> MSSNRVLDLFKPFESFLPEVIAPERKVPYNQKLIWTGVSLLIFLILGQIPLYGIVSSETSDPLYWLRAMLASNRGTLLELGVSPIITSSLIFQFLQGTQLLQIRPESKQDRELFQIAQKVCAIILILGQALVVVMTGNYGAPSDLGLPICLLLIFQLMFASLIVMLLDELLSKGYGLGSGISLFIATNIAEQIFWRAFAPTTVNSGRGKEFEGAVIAFFHLLAVRKDKKRALVEAFYRTNLPNMFQVLMTVAIFLFVLYLQGFRYELPIRSTKVRGQIGIYPIKLFYTSNTPIILQSALTSNIFLISQILFQKYPTNPLIRLIGVWGIRPGTQGPQMALSGLAYYIQPLMSLSEALLDPIKTIVYITFVLGSCAVFSKTWIEISGTSPRDIAKQFKDQGMVINGKRETSIYRELKKIIPTAAAFGGATIGALSVGSDLLGTLGSGASILLATTTIYGYYEAAAKEGGFTKNLVPGFSDLM;> MSSPTPPGGQRTLQKRKQGSSQKVAASAPKKNTNSNNSILKIYSDEATGLRVDPLVVLFLAVGFIFSVVALHVISKVAGKLF;> MARASEKGEEKKQSNNQVEKLVEAPVEFVREGTQFLAKCKKPDLKEYTKIVKAVGIGFIAVGIIGYAIKLIHIPIRYVIV;> GGSGGSGGSGGSGGSPTNYEYDEASETWPSFILTGLLMVVGPMTLLQIYQIFFGANAEDGNSGKSKEFNEEVFKNLNEEYTSDEIKQFRRKFDKNSNKKSKIWSRRNIIIIVGWILVAILLQRINSNDAIKDAATKLFDPYEILGISTSASDRDIKSAYRKLSVKFHPDKLAKGLTPDEKSVMEETYVQITKAYESLTDELVRQNYLKYGHPDGPQSTSHGIALPRFLVDGSASPLLVVCYVALLGLILPYFVSRWWARTQSYTKKGIHNVTASNFVSNLVNYKPSEIVTTDLILHWLSFAHEFKQFFPDLQPTDFEKLLQDHINRRDSGKLNNAKFRIVAKCHSLLHGLLDIACGFRNLDIALGAINTFKCIVQAVPLTPNCQILQLPNVDKEHFITKTGDIHTLGKLFTLEDAKIGEVLGIKDQAKLNETLRVASHIPNLKIIKADFLVPGENQVTPSSTPYISLKVLVRSAKQPLIPTSLIPEENLTEPQDFESQRDPFAMMSKQPLVPYSFAPFFPTKRRGSWCCLVSSQKDGKILQTPIIIEKLSYKNLNDDKDFFDKRIKMDLTKHEKFDINDWEIGTIKIPLGQPAPETVGDFFFRVIVKSTDYFTTDLDITMNMK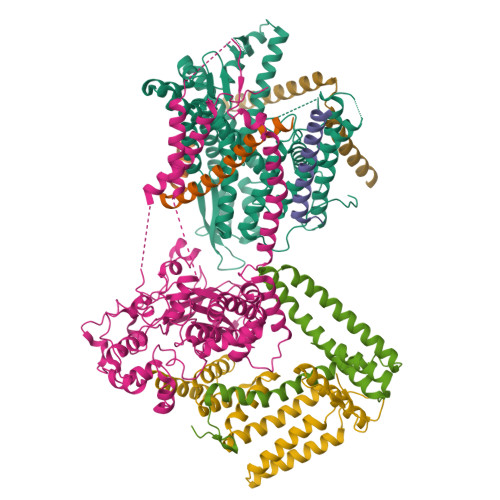VRDSPAVEQVEVYSEEDDEYSTDDDETESDDESDASDYTDIDTDTEAEDDESPEAGGATTASGTGENLYFQ;> MSEFNETKFSNNGTFFETEEPIVETKSISVYTPLIYVFILVVSLVMFASSYRKKQAKKISEQPSIFDENDAHDLYFQIKEMSENEKIHEKVLKAALLNRGAESVRRSLKLKELAPQINLLYKNGSIGEDYWKRFETEVKLIELEFKDTLQEAERLQPGWVQLFVMVCKEICFNQALSRRYQSILKRKEVCIKEWELKINNDGRLVN;> MVTLEYNANSKLITASDAVVALSTETNIDQINVLTTSLIGETNPNFTPQPNEALSKMIKGLFESGMKNLQQKKLNEALKNVSLAIEMAQRKRAPWEAFAIQLPELHFMLRSKIDLCLILGKHLEALQDLDFLLGTGLIQPDVFVRKADCLLKLRQWEEARATCERGLALAPEDMKLRALLIETARNLAEYNGE> MSLGQTTLACSFRSLTNPYYTAFNKGAQSFAKSVGLPYVPLTTEGSSEKGIADIRALLQKTGGNLVLNVDPNDSADARVIVEACSKAGAYVTTIWNKPKDLHPWDYNPNYVAHLSYDGVAYGEETATQLFKSMGGKGGVVALGGIFSNVPAIERKAGLDAALKKFPGIQLLDFQVADWNSQKAFPIMQAWMTRFNSKIKGVWAANDDMALGAIEALRAEGLAGQIPVTGMDGTQPGLVAIKSGELVASVDWDPFWLGGIGLSMGLQAKEKKIDLA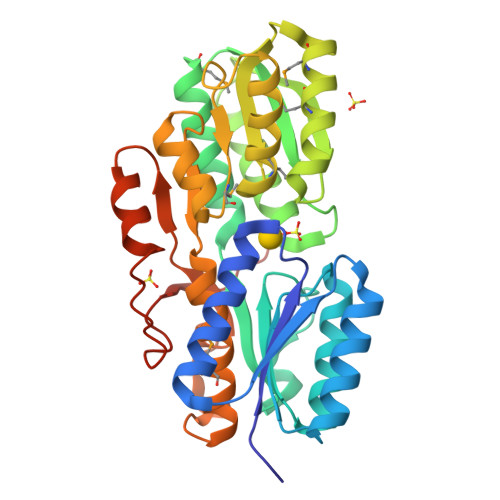TLPKDRRESFCTATFVTKTNVQDVIARAASPKAEWNNLYARVAGPVVYREGHHHHHH> MEDKTLIKKRIDWFCKNKINAFSPTISPAPKSVERNEIESLYEGILWFVLNGVKEIVIEKKYMGSYCDIYLHRRLEDTYLVSRNGYKINHLDQEQCLRALQGLHDRFSWDGVELRIIQSELMPWSILGKGLINNEFSAYYISHEIHAEYLVQSSLYEKLQKIQQEPAYLSFVADAKVLSAKELKDKYPMHIIRQYQSIRDFKFLDLPHYQQNIQLFKRQLDIFGKEAAPFFKPFNILKEVYTDGREHFVNDNLSFQQINDDDFLHYQFTDREDFEAKYPQI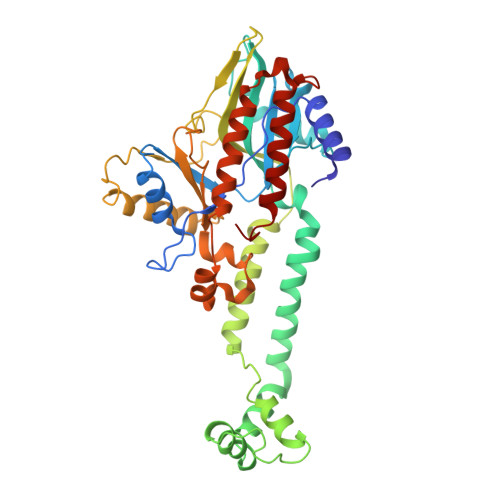RAWVDQVNQSDEEGVVIKPRTAFLPGMPPAFKVRNNDYLTLVYGVDFEDRLQEQIAKRNIKGKLRCSINDWAINAKLLAIPYSELGEENYELKNLVLDRILGEEIENQLDSRL>TGCVLNKLFQLPTPPLSRHQLKRLEEHRYQSAGRSLLEPLMQGYWEWLVRRVPSWIAPNLITIIGLSINICTTILLVFYCP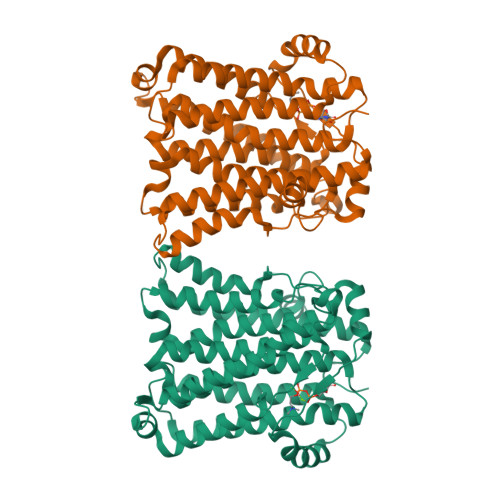TATEQAPLWAYIACACGLFIYQSLDAIDGKQARRTNSSSPLGELFDHGCDSLSTVFVVLGTCIAVQLGTNPDWMFFCCFAGTFMFYCAHWQTYVSGTLRFGIIDVTEVQIFIIIMHLLAVIGGPPFWQSMIPVLNIQMKIFPALCTVAGTIFSCTNYFRVIFTGGVGKNGSTIAGTSVLSPFLHIGSVITLAAMIYKKSAVQLFEKHPCLYILTFGFVSAKITNKLVVAHMTKSEMHLHDTAFIGPALLFLDQYFNSFIDEYIVLWIALVFSFFDLIRYCVSVCNQIASHLHIHVFRIK[2x]Microtubule (MT) nucleation is regulated by the γ-tubulin ring complex (γTuRC), conserved from yeast to humans. In budding yeast, homologues of the grip-containing proteins (GCPs) GCP2 and GCP3 (Spc97p and Spc98p) and two copies of γ–tubulin (Tub4p) form a 300 kDa complex (γTuSC). Spc110p, a distant pericentrin homologue, recruits this complex to the nuclear face of the spindle pole body (SPB), while Spc72p recruits it to the cytoplasmic face. In yeast, the CM1 motif is required for seven identical γTuSCs to helically assemble into a γTuRC at the SPB.

Motivated by the crosslinks observed between the Spc110pNCC and γTuSC, we sought a higher-resolution structure of the NCC region via X-ray crystallography. Previous work indicated that Spc1101-220 is only weakly dimeric. Using the proven strategy of fusing weakly interacting coiled-coils with stabilizing domains, we found that an N-terminal fusion of Spc110p164-207 with a domain from Xrcc4 produced high yields of soluble protein. The Xrcc4-Spc110p164-207 construct crystallized in a variety of conditions, diffracted to 2.1 Å, and enabled phases to be obtained by molecular replacement using Xrcc4 as a search model. As expected, the electron density map was consistent with a coiled-coil, with interpretable density for Spc110p164-203 residues. When the coiled-coil was docked into the 6.9 Å cryo-EM map using cross-correlation in Chimera, the X-ray model occupied most of the alpha-helical cryo-EM density. Importantly in the docked conformation the majority of the unique crosslinks were satisfied. Given the observed pitch of the coiled-coil in the crystal structure, as well as density for larger side chains, we were able to assign the register of the NCC. We observed a significant number of crosslinks between the N-terminal portions of Spc97p and Spc110pNCC. Thus, this region and not CM1 was responsible for the coiled-coil-γTuSC interaction apparent in the cryo-EM map.

>GPGSGGSGERKISRIHLVSEPSITHFLQVSWEKTLESGFVITLTDGHSAWTGTVSESEISQEADDMAMEKGKYVGELRKALLSGAGPADVYTFNFSKESCYFFFEKNLKDVSFRLGSFNLEKVENPAEVIRELICYCLDEIKSLKHEIKELRKEKNDTLNNYDTLEEETDDLKNRLQALEKEL[2x]> YT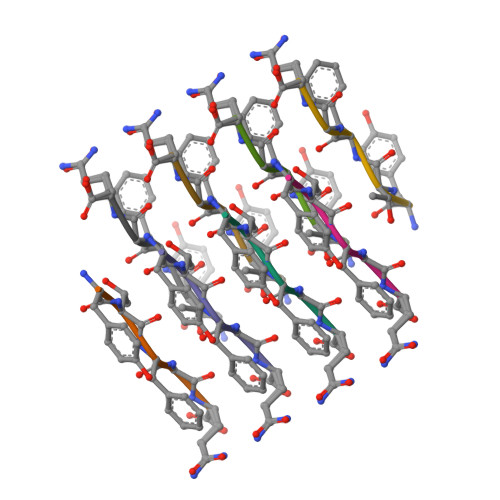FGQ> MDINGG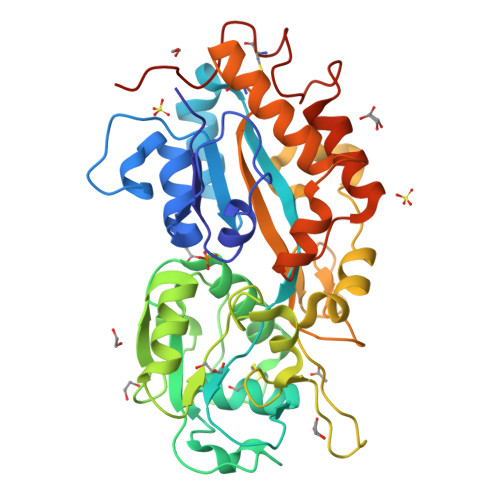GATLPQALYQTSGVLTAGFAQYIGVGSGNGKAAFLNNDYTKFQAGVTNKNVHWAGSDSKLSATELSTYASAKQPTWGKLIQVPSVGTSVAIPFNKSGSAAVDLSVQELCGVFSGRINTWDGISGSGRTGPIVVVYRSESSGTTELFTRFLNAKCNAETGNFAVTTTFGTSFSGGLPAGAVAATGSQGVMTALAAGDGRITYMSPDFAAPTLAGLDDATKVARVGKNVATNTQGVSPAAANVSAAIGAVPVPAAADRSNPDAWVPVFGPDNTAGVQPYPTSGYPILGFTNLIFSQCYADATQTTQVRDFFTKHYGASNNNDAAITANAFVPLPTAWKATVRASFLTASNALSIGNTNVCNGIGRPLLEHHHHHH>NGFRLNHVPYVSQQNERMGCWYACTRMLGHSISSGPRLGLPEL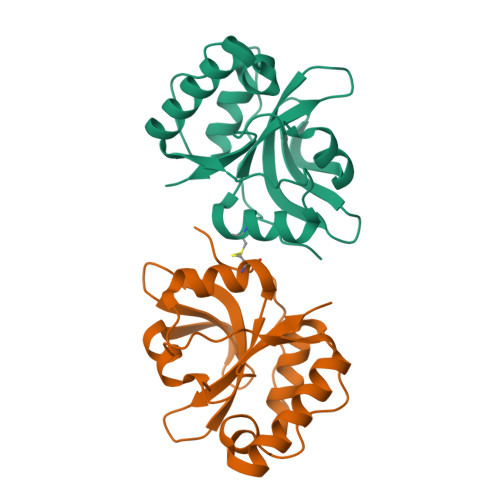YDSSGPQGLQQREDVLRLMRNENLAEVSLPESRQFSANELGNLLCRHGPIMFGWQTPAGSWHMSVLTGIDKPNDAIIFHDPQRGPDLTMPLDSFNQRLAWRVPHAMLYSEN[2x]>[2x]LLPVKYCKMRIFSGSTAAAPEEEPFEVWLEQATEIAKEWPIPEAEKKRWVAESLRGPALDLMHIVQ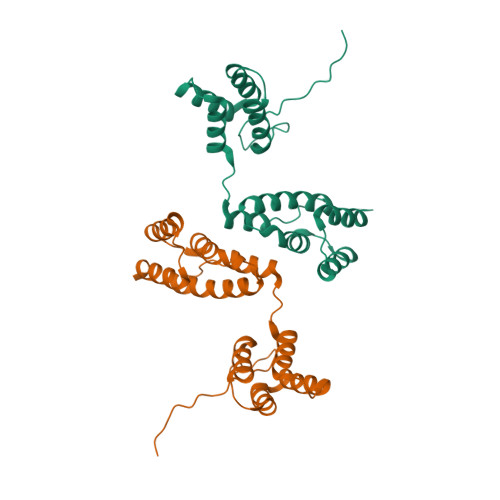ADNPSISVGECLEAFKQVFGSTESRRTSQVKYLRTYQQEGEKISAYVLRLETLLRRAVEKRAIPRNIADQVRLEQVMAGANLGNVLWCRLQELKDQGPLPTFLQLMKVIREEEE>GMIKKEGPGWRIIFDSSRDNFSTLIGGETWAIELDKSEWKILVEVVMELCDQYKLVKEQL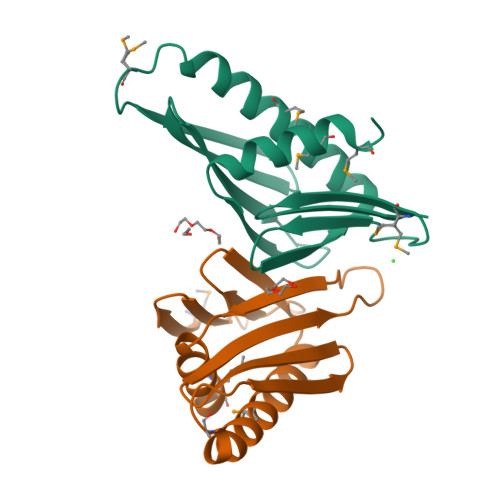MGDEDITLELERRPWLAILNGDQYGWNLRLILSASGLFNRGAEVYWPRHVTNNVVNAMRSMWDSDYL[4x]>[6x]MTAVETKKQYLTVFKEDGIAEIHLHINKSNSYDLEFYKEFNAAIDDIRFDPDIKVVIVMSDVPKFFSAGADINFLRSADPRFKTQFCLFCNETLDKIARSPQVYIACLEGHTVGGGLEMALACDLRFMGDEAGKIGLPEVSLGVLAGTG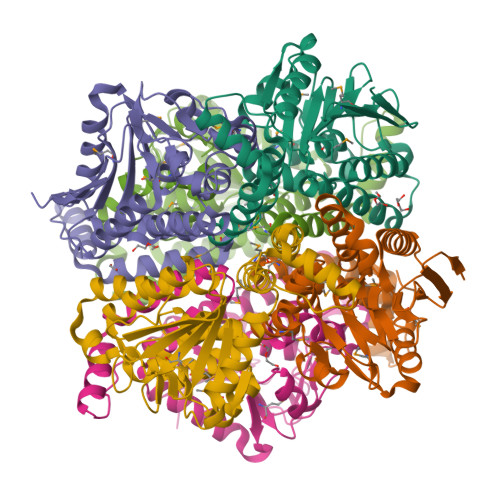GTQRLARLIGYSRALDMNITGETITPQEALEIGLVNRVFPQAETRERTREYARKLANSATYAVSNIKLAIMNGKEMPLNVAIRYEGELQNLLFRSEDAKEGLSAFLEKRQPNWKGI>GPAVPRMVVLHSLLGMAVLIAIAVLLSTDRKAINIRTVAGAFLIQVALGALVLYVPQGRDMLGEASKTISNVIAYGNNGVDFLFGGLVSEKMFEVFGGGGFVFALRVLPMIVFFSSLMAVLYYIGVMQLLIKVIGGFLQKMLGTSKAESMSAAALIFVGQTEAPLVVRPYIRRMTE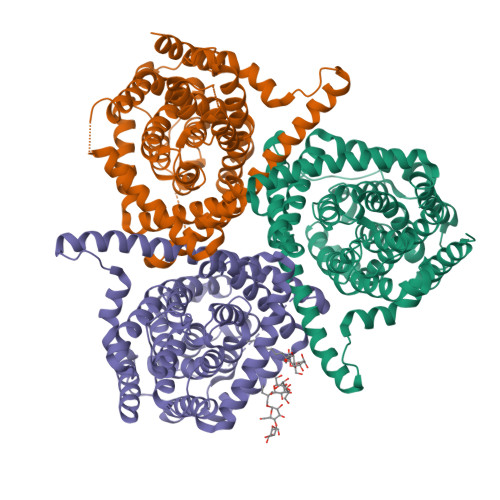SELFAVMSGGLASVAGSVLAGYVQMGVPLPYLIAASFMAAPGGLLFAKLLVPETERTQNDAEVLAENEDEKPTNVIDAAASGAVTGAQIAIAVGASLLAFVALIAMINGIIGGVGGWFGHGDLTLQAILGWLFSPLAWVIGVPWSEAGIAGSLIGQKVVINEFVAYSEFVKYLKPEAAVQLSDTTKAIISFALCGFANLGSIAVLVGGLSIMAPKRRKDVARLGIKAVVAGSLSNLMSAVIAGLFTGLSGASVLG[3x]2,3,4,6,8-PENTACHLORO-9H-CARBAZOL-1-OL 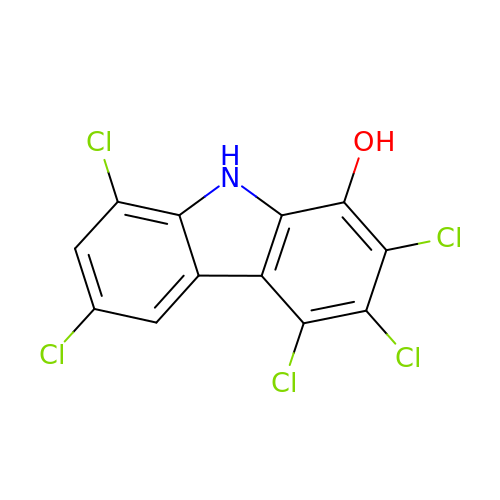| C12 H4 Cl5 N O | AEMWOCRPUWTJCH-UHFFFAOYSA-N> GSHMEEVSEYCSHMIGSGHLQSLQRLIDSQMETSCQITFEFVDQEQLKDPVCYLKKAFLLVQDIMEDTMRFRDNTPNAIAIVQLQELSLRLKS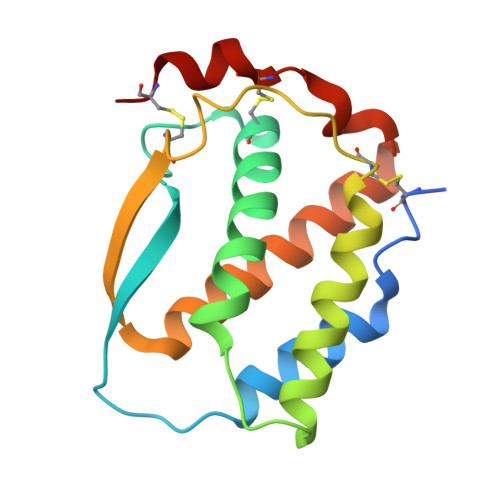CFTKDYEEHDKACVRTFYETPLQLLEKVKNVFNETKNLLDKDWNIFSKNCNNSFAECSSQ>[8x]MRTRIFIGSSKEGLKEANYVKSRLEKANFEVFIWNDDIFKPNKNTLETLLNVASLFDFGIMIATKDDFTASRDDIFETVRDNVVFEFGLFLGRLGENRAFALQENGAKLPSDLLGITIPKFEKTDDYFSNYNLNTEIDNIIKII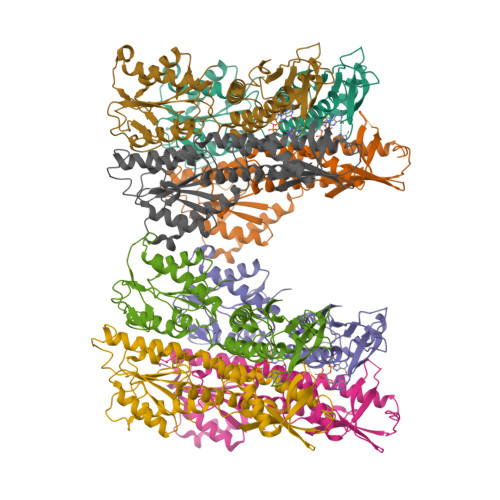NEKISLGELGLLPSTVLAIGYYENFVSTVCDALHSLPTIKLNGIEYKDFVFNIIIPNDLDADIKRRAQIYFKKMDIHEVKIDTNGRSFPLYLQIDEENSGDVAVLYDMPTTLGGIDKAIEMYMKKGHIGKTSQQQLLEERELRNFKTTLINLINNNSFTKTFVKVIEE> GNDDPGKDPDVVTYDFKNLPADSGAKPTEDQMSAVVATFVDEVALPTYKDMLTKMTAYKNAVDKFIASGSKNDLADACDAWRAVRVPWEQSEAFLFGVADLAQLDPSLDSWPLDKNGIEEIIATGEFSKISGAVDEDAEDGPQNLRGFHTAEKMLFLDGEPRDLETSPFAKNELEYLKLVSERMLSDTQDLYNGWLKGLGTSDVPSSYAEAMKKHDGSAYSIGNVYQAIELMLN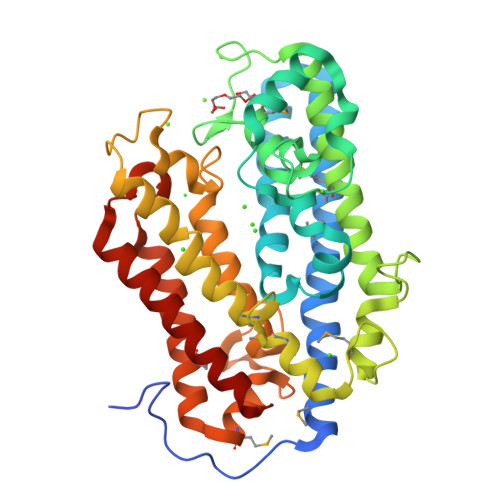GNNGMAGISNEVGSAKITDPVTAWNGSNKDATDPNNPGVLAVESWYSWNSLDDYKNNIVSIKNAYFGGRDLDEESASESSLHALTKMINPTLDSLMVVQIDKTIDAINAIGYPFRNNLGDTEHINTATEACADLTTGLGVVKSKFTN>[2x]GNENPDKPTDDVNYNMNEPRLASTLRGGLIIEGNVEQRLKPLQIDFYSQMTVDGGGWGTKNYIQD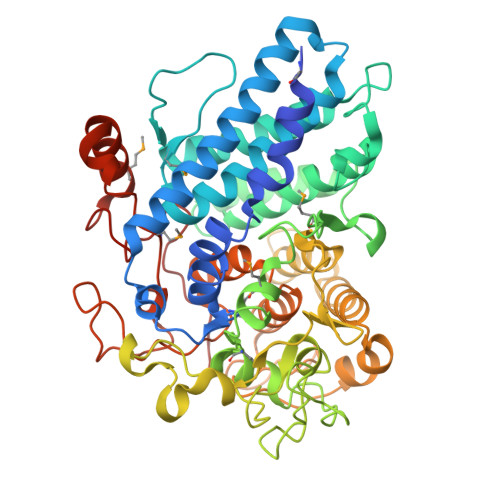DEWNNLVWEEYLKQIASINIVIRSLTEKDKDAYANTIAFARIWRVYVHTLAADKFGPMPFPAYEIVEANPPYKSLKDIYDEYFRELDAAINGFNDSAQPIFSDAGIDLIYKNDVSKWKRFANSLRLRLAVRLTEVDQEKCIAEANAAISSPAGLISDKADNAYMPPKADGSWGQDYNYTMFQITWSGPICMSKSVEKLVTNIGGVAWPQGVVNQTSGVAVSSVHPEKVDPRAPKIFQPGIENGDWKGLVYGPKAEEANTGIYQSKQCAELGFIIKDGYPYKSRPYDLFLSEEVHFLKAELYARGFIAGDAKSEYEAGVRASFATWGVTSEVDDYLTSTEKNEAGTSARYDDQQGAGNTALEKIITQKYIAGIPDLAQEGWNDKRRLNLPRLDVAVYRDQAVYNNNDKDILKSANFIKRMRYPTKESLINATEYEKGKSMLGGKGDIVSTPLWWDKNSNYCTSSK> GDKAYTDAESYTKGLHKIYSVWALSGQDGSSSSDISGLDAGNTALLRCWWTLQEQPT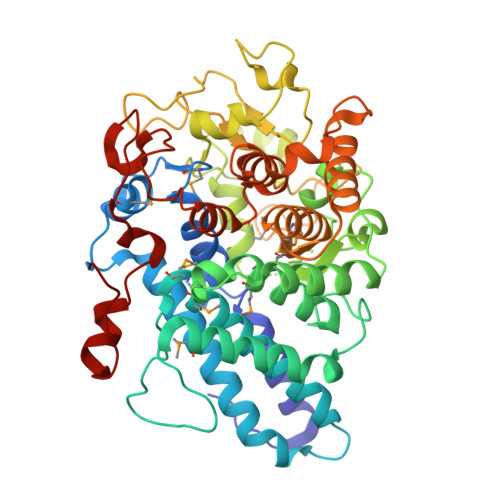DEMKNAWNDAWCTEVNYMTWTTNKVEPIEGVYQRCMYIVALVNEFLKNIPNAPESIDKESYIAQARFNRAFAYYVLMDMFALPPFITEKNYSIEPAPLSREDLFNWIEAELNEIKPNLPSPRSEYGVADQAVASALLARMYLNAEIYTGKARYTECINACNEVIKAGYQLADNYADLFKADNGENPDTKKEIIYPIIFDGDKTQSWGMAAIIIGARGAEDKDVLLAHSGVDQGWAGFRATSNLVHLFDFQNDEEPKASEIQDKRGIFYDKGRSIDITSSVSGTFETEGWSVFKFSNLNSNGQPGKNTLWVDTDFPMFRLGDIYLMYAEAVARGGEGSKASAVEYINALRKRAYGDDKHNISENWLEENNFRNLLDERGRELYWEGIRRTDLVRFDLLTSGSYTWDFKGGINTGVGVNKRYNVYPIPVTDLTVNGNLQQNEGY Retinoid X receptor α (RXRα), a member of the nuclear receptor superfamily and a validated drug target, exists in different oligomeric forms that regulate a broad spectrum of cellular processes under both physiological and pathophysiological conditions. Like other nuclear receptors, RXRα comprises an intrinsically disordered N-terminal A/B domain with poorly defined functions, a central DNA-binding domain (DBD), and a ligand-binding domain (LBD) in which α-helices are arranged around a central hydrophobic ligand-binding pocket (LBP). A unique property of RXRα is an auto-repressive mechanism involving homotetramerization, in which a ‘dimer-of-dimers’ pack in a bottom-to-bottom manner, with H12 from each monomer invading (and invaded by) a neighbouring domain across the tetramer interface. The equilibrium between inactive homotetramers and active homodimers is tightly regulated by ligand binding.

To understand how K-80003 modulates the biological activity of tRXRα, we determined the crystal structure of RXRα-LBD in complex with K-80003 to a resolution of 2.6 Å. We found that the RXRα-LBD/K-80003 complex adopts a tetrameric structure, similar to those observed in crystals of apo-RXRα or RXRα-LBD/tRA-isomer complex, in which two RXRα-LBD canonical homodimers (labelled A1/B1 and A2/B2) pack in a bottom-to-bottom manner with point group symmetry D2. Besides the canonical dimer interface, there are two symmetry-related interfaces involving subunits A1/B2 and B1/A2. These ‘tetramer’ interfaces comprise three sub-regions: parallel packing between symmetry-related H3 helices; ‘end-to-end’ packing between H11 that reduces their length by two helical turns (compared with the agonist-bound structure); and the invasion of each H12 helix into its apposing domain, where it binds to the coregulator-binding groove, consisting of elements of H3 and H4. Refinement of the structure and careful inspection of difference Fourier maps revealed six molecules of K-80003-bound per tetramer, with three molecules per A1/B2 or A2/B1 interfacial cavity. The 2 A1/B2 and A2/B1 interfacial cavities are symmetry-related and the three bound molecules in each cavity (K-80003A, K-80003B and K-80003C, respectively) appear to play distinct but complementary roles in stabilizing the tetramer. Thus, K-80003A and K-80003B are arranged about the A1/B2 pseudo-dyad, making similar but distinct interactions. They bind in a region where the H12 is located in the agonist-bound RXRα-LBD structure and thus distinct from the canonical ligand-binding region.

>GSHMTSSANEDMPVERILEAELAVEPKTETYVEANMGLNPSSPNDPVTNICQAADKQLFTLVEWAKRIPHFSELPLDDQVILLRAGWNELLIASFSHRSIAVKDGILLATGLHVHRNSAHSAGVGAIFDRVLTELVSKMRDMQMDKTELGCLRAIVLFNPDSKGLSNPAEVEALREKVYASLEAYCKHKYPEQPGRFAKLLLRLPALRSIGLKCLEHLFFFKLIGDTPIDTFLMEMLEAPHQMT[4x]> MEIVSKLTLKTIGAQPKPHSVKENTALASIYGRVRGKKVGQSTFGDFIKFEGEFEGVNIATGEVFRSGALILPKVLESLLAGAVDGENTVDFAVEIWAKPSEKGNTGYEYGVKPLIEPAASDELAALRNQVKAALPAPAAAG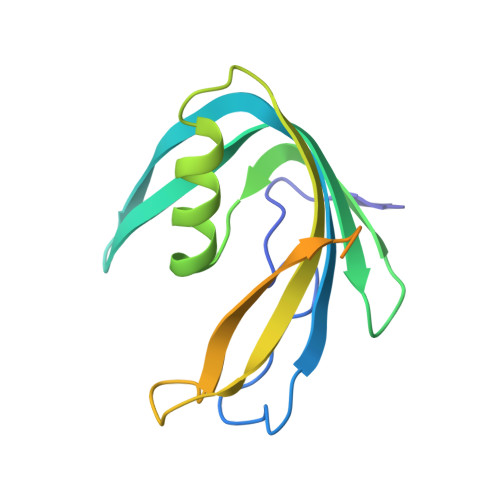EAAAEAKPAAKAKAKAEA>TLIELMIVVAIIGILAAIAIPQYQNYIAKSQVSRVMSETGSLKTVIETCI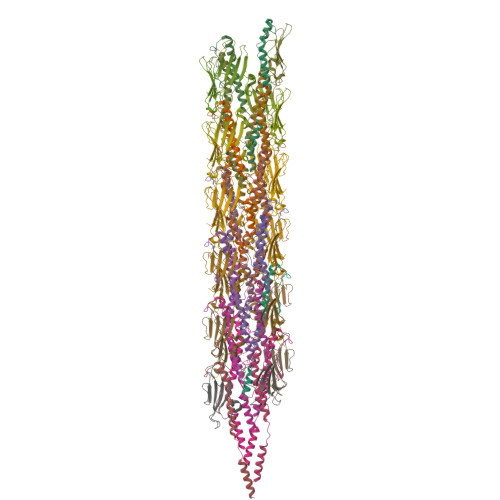LDGKTAANCELGWTNSNLLG[22x];>STAAVTGQTGLTITYPASATESAAIQGTFGNSAAIKIKNQTLTWTRTPEGAWSCATTVEAKFKPAGCAS[22x]piperidine-2,6-dione | C5 H7 N O2 | 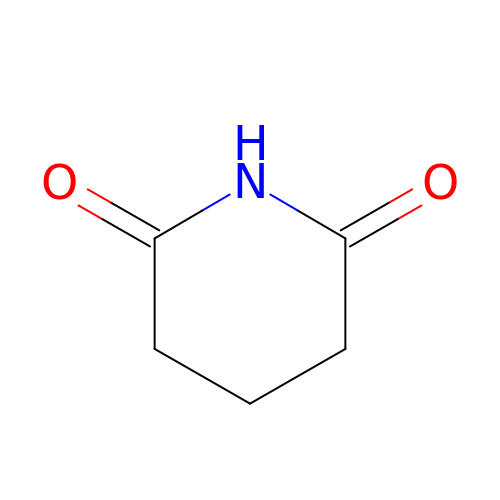KNCYXPMJDCCGSJ-UHFFFAOYSA-N>GSSGSSGMQIGKIIKVSGPLVMAENMSEASIQDMCLVGDLGVIGEIIEMRQDVASIQVYEETSGIGPGEPVRSTGEALSVELGPGIISQMFDGIQRPLDTFMEVTQSNFLGRGVQLPALDHEKQWWFEATIEEGTEVSAGDIIGYVDETKIIQHKIMVPNGIKGTVQKIESGSFTIDDPICVIETEQGLKELTMMQKWPVRRGRPIKQKLNPDVPMITGQRVIDTFFPVTKGGAAAVPGPFGAGKTVVQHQIAKWSDVDLVVYVGCGERGNEMTDVVNEFPELIDPNTGESLMERTVLIANTSNMPVAAREASIYTGITIAEYFRDMGYDVAIMADSTSRWAEALREMSGRLEEMPGDEGYPAYLGSRLAEYYERSGRVIALGSDQREGSITAISAVSPSGGDISEPVTQNTLRVVKVFWGLDSSLAQKRHFPSINWIQSYSLYSTEVGRYMDQILQQDWSDMVTEGMRILQEEEQLNEIVRLVGIDSLSDNDRLTLEVAKSIREDYLQQNAFDDVDTFTSREKQFNMLKVILTFGKEARKALSLGAYFNEIMEGTVAVRERISRSKYIPEEELAKISSINEEIKETIQLIVSEGGMTDD[3x];>[3x]GSSGSSGMIKEYRTIKEVVGPLMAVEKVSGVKYEELIEVRMQNGEIRRGQVLEVQEDKAMVQIFEGTSGINLKNSSVRFLGHPLQLGVSEDMIGRVFDGLGRPKDNGPEILPEKYLDINGEVINPIARDYPDEFIQTGISAIDHLNTLVRGQKLPVFSGSGLPHKELAAQIARQATVLDSSDDFAVVFAAIGITFEEAEFFMEDFRQTGAIDRSVMFMNLANDPAIERIATPRMALTAAEYLAYEKGMHVLVIMTDMTNYAEALREISAARREVPGRRGYPGYLYTNLATLFERAGRIRGLKGSVTQIPILTMPEDDKTHPIPDLTGYITEGQIILTRELYKSGIQPPIDVLPSLSRLKDKGTGAGKTREDHAATMNQLFAAYAQGKQAKELAVVLGESALSDIDKIYAKFAERFENEYVNQGFYTNRTITETLDLGWELLAMLPRTELKRIKDDLLDKYLPEGK;> GSSGSSGMRLNVNPTRMELTRLKKQLTTATRGHKLLKDKQDELMRQFILLIRKNNELRQAIEKETQTAMKDFVLAKSTVEEAFIDELLALPAENVSISVVE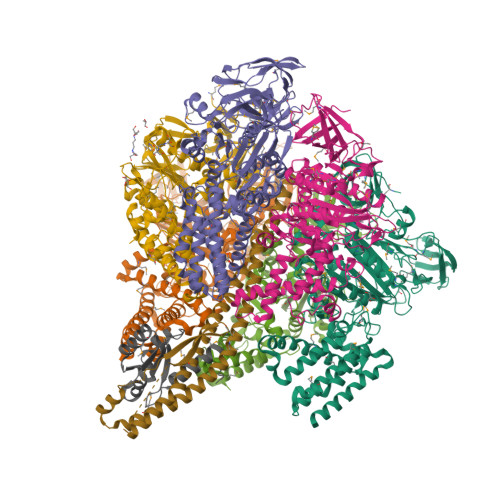KNIMSVKVPLMNFQYDETLNETPLEYGYLHSNAELDRSIDGFTQLLPKLLKLAEVEKTCQLMAEEIEKTRRRVNALEYMTIPQLEETIYYIKMKLEENERAEVTRLIKVKNMGTEE;> MTYKIGVVGDKDSVSPFRLFGFDVQHGTTKTEIRKTIDEMAKNEYGVIYITEQCANLVPETIERYKGQLTPAIILIPSHQGTLGIGLEEIQNSVEKAVGQNILSGPSSGENLYFQ> MKDLLKFLKAQTKTEEFDAIKIALASPDMIRSWSFGEVKKPETINYRTFKPERDGLFCARIFGPVKDYECLCGKYKRLKHRGVICEKCGVEVTQTKVRRERMGHIELASPTAHIWFLKSLPSRIGLLLDMPLRDIERVLYFESYVVIEGGMTNLERQQILTEEQYLDALEEFGDEFDAKMGAEAIQALLKSMDLEQECEQLREELNETNSETKRKKLTKRIKLLEAFVQSGNKPEWMILTVLPVLPPDLRPLVPLDGGRFATSDLNDLYRRVINRNNRLKRLLDLAAPDIIVRNEKRMLQEAVDALLDNGRRGRAITGSNKRPLKSLADMIKGKQGRFRQNLLGKRVDYSGRSVITVGPYLRLHQCGLPKKMALELFKPFIYGKLELRGLATTIKAAKKMVEREEAVVWDILDEVIREHPVLLNRAPTLHRLGIQAFEPVLIEGKAIQLHPLVCAAYNADFDGDQMAVHVPLTLEAQLEARALMMSTNNILSPANGEPIIVPSQDVVLGLYYMTRDCVNAKGEGMVLTGPKEAERLYRSGLASLHARVKVRITEYEKDANGELVAKTSLKDTTVGRAILWMIVPKGLPYSIVNQALGKKAISKMLNTCYRILGLKPTVIFADQIMYTGFAYAARSGASVGIDDMVIPEKKHEIISEAEAEVAEIQEQFQSGLVTAGERYNKVIDIWAAANDRVSKAMMDNLQTETVINRDGQEEKQVSFNSIYMMADSGARGS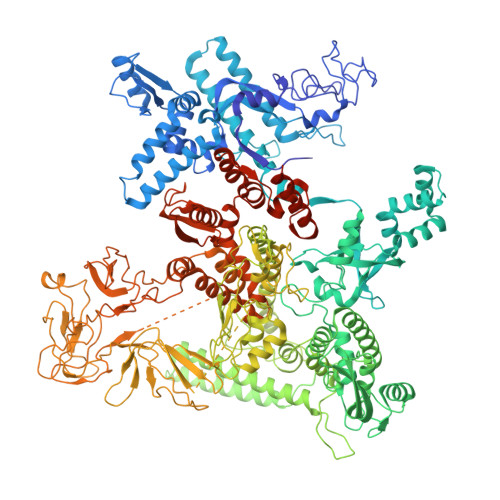AAQIRQLAGMRGLMAKPDGSIIETPITANFREGLNVLQYFISTHGARKGLADTALKTANSGYLTRRLVDVAQDLVVTEDDCGTHEGIMMTPVIEGGDVKEPLRDRVLGRVTAEDVLKPGTADILVPRNTLLHEQWCDLLEENSVDAVKVRSVVSCDTDFGVCAHCYGRDLARGHIINKGEAIGVIAAQSIGEPGTQLTMRTFHIGGAASRAAAESSIQVKNKGSIKLSNVKSVVNSSGKLVITSRNTELKLIDEFGRTKESYKVPYGAVLAKGDGEQVAGGETVANWDPHTMPVITEVSGFVRFTDMIDGQTITRQTDELTGLSSLVVLDSAERTAGGKDLRPALKIVDAQGNDVLIPGTDMPAQYFLPGKAIVQLEDGVQISSGDTLARIPQESGGTKDITGGLPRVADLFEARRPKEPAILAEISGIVSFGKETKGKRRLVITPVDGSDPYEEMIPKWRQLNVFEGERVERGDVISDGPEAPHDILRLRGVHAVTRYIVNEVQDVYRLQGVKINDKHIEVIVRQMLRKATIVNAGSSDFLEGEQVEYSRVKIANRELEANGKVGATYSRDLLGITKASLATESFISAASFQETTRVLTEAAVAGKRDELRGLKENVIVGRLIPAGTGYAYHQDRMRRRAAGEAPAAPQVTAEDASASLAELLNAGLGGSDNELERRASENLYFQGHHHHHHHHHH>SMEETIRKGSEVEVSSTEEGFADAWFRGILQENPTKSGRKKLRVRYLTLLNDDALSPLIENIEPRFIRPVPPENEYNGIVLEEGTVVDADHKDGWWTGVIIKKLENGKFWVYYDSPPDIIEFERNQLRPHLRWSGWKWLRPDIQELDKSMFSSGTMAEVSTIVDKAEVAWFPAMIIKEIEVDGEKKFIVKDCNKHLSFSGDEARTNSTIDSSRVRPTPPPFPVEKYELMDRVEVFRGSVWRQGLVRGVLDHNCYMVC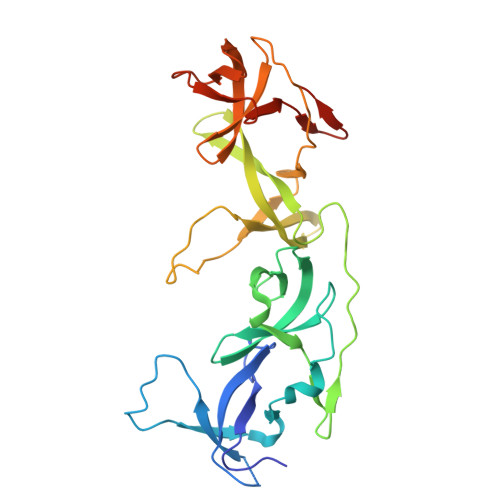LVVTAAAPVVKHSDLRPCKVWEDGQTPVIETPSN[2x]> MEMPICAFQLPDLTVYNEDFRSFIERDLIEQSMLVALEQAGRLNWWVSVDPTSQRLLPLATTGDGNCLLHAASLGMWGFHDRDLMLRKALYALMEKGVEKEALKRRWRWQQTQQNKESGLVYTEDEWQKEWNELIKLASSEPRMHLGTNGANCGGVESSEEP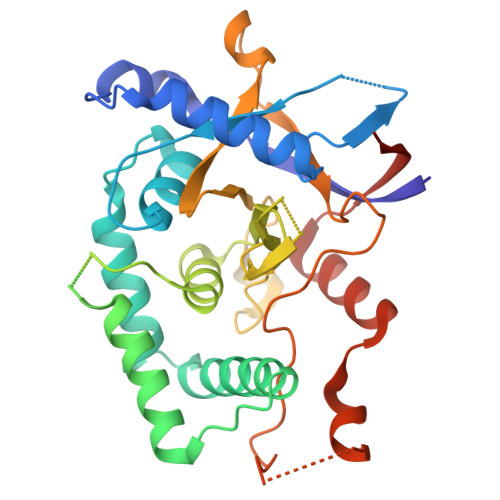VYESLEEFHVFVLAHVLRRPIVVVADTMLRDSGGEAFAPIPFGGIYLPLEVPASQCHRSPLVLAYDQAHFSALVSMEQKENTKEQAVIPLTDSEYKLLPLHFAVDPGKGWEWGKDDSDNVRLASVILSLEVKLHLLHSYMNVKWIPLSSKHHHHHH Here, we focus on the mucin-selective metalloprotease, Amuc_0627 (AM0627), which is known to cleave between adjacent residues carrying truncated core 1 O-glycans. We showed that this enzyme is capable of degrading purified mucin 2 (MUC2), the major protein component of mucus in the gut. Of the enzymes characterized to date, AM0627 from A. muciniphila is unique in its strict requirement for adjacent O-glycosylated residues. The M60-like or Pfam 13402 (PF13402) family consists of hundreds of enzymes from organisms known to inhabit mucosal host environments.

To probe the molecular basis for O-glycan specificity, we determined the structure of AM0627 in its unliganded form, with the signal peptide (residues 1–20) removed, at 1.9 Å resolution via X-ray crystallography. AM0627 consists of an immunoglobulin-like fold domain followed by a catalytic domain. The active site harboring catalytic residue E326 contains a beta strand and two alpha helices arranged within the larger gluzincin motif, characterized by histidine residues H325 and H329 and glutamate residue E343 bound to a zinc ion. Sequence alignments of AM0627 with active, structurally characterized PF13402 enzymes highlighted conserved tryptophan, glycine, asparagine/glutamine, and arginine residues that interact with the initiating α-GalNAc of mucin-type O-glycans, as exemplified by a cocrystal structure obtained by Noach et al. of BT4244 with a serinyl Tn antigen. Notably, these S1′ subsite residues are spatially conserved between AM0627, BT4244, ZmpB, ZmpC, and IMPa, providing a rationale for the specificity of these proteases for substrates carrying mucin-type O-glycosylation, a property that may be shared by the entire PF13402 family. The active site beta strand is positioned further from the gluzincin motif residues in AM0627 compared to related enzymes, preventing the formation of hydrogen bonds typically observed between metallopeptidases and their ligands. Comparison of the catalytic helices between PF13402 enzymes revealed that AM0627 and BT4244 have longer helices containing a spatially conserved aspartate residue. This residue, together with a semiconserved Y288, forms a surface that sterically blocks accommodation of a G2′ sugar residue. Notably, a cluster of aromatic residues, formed by a nonconserved W149 present in a long loop as well as residues Y287 and F290 in and around the active site beta strand, was observed adjacent to the active site. Unique to AM0627 was the presence of a long loop that, based on molecular docking, could interact with a glycan at the P1 position via formation of a hydrophobic pocket consisting of residues W149, Y287, and F290.

> MANTPEHIGNDLKLFKDSSCTSLKPDVKNTSAFQSDAMKELATKILAGHYKPDYLYAEYRALPSPRQTGKNLRIGDGFSKYDNMTGVYLEKGRHVVLVGKTEGQEISLLLPNLMRKPAEGVQPTKDPNGWGLHKKQIPLKEGINIIDVETPANAYISYFTEDAGKAPKIPVHFVTGKANGYFDTTRGDTNKDWVRLLDQAVSPIMDARGKYIQVAYPVEFLKKFTKDRGTELINAYDKLIGIQYQLMGLDKYGKIPENRVLARVNFNYYMFRDGDGVAYLGNDGTMRMVTDPENVLKGDACWGFSHEVGHVMQMRPMTWGGMTEVSNNIFSLQAAAKTGNESRLKRQGSYDKARKEIIEGEIAYLQSKDVFNKLVPLWQLHLYFTKNGHPDFYPDVMEYLRNNAGNYGGNDTVKYQFEFVKACCDVTKTDLTDFFEKWGFFKPGKFHIGDYAQYDFNVTPEMVEETKKWIAGKGYPKPETDITELSE>MNHKVHHHHHHMELGTLEGSENLYFQGAMARGVNKVILIGNLGDKPELRYTGSGTAVCNMS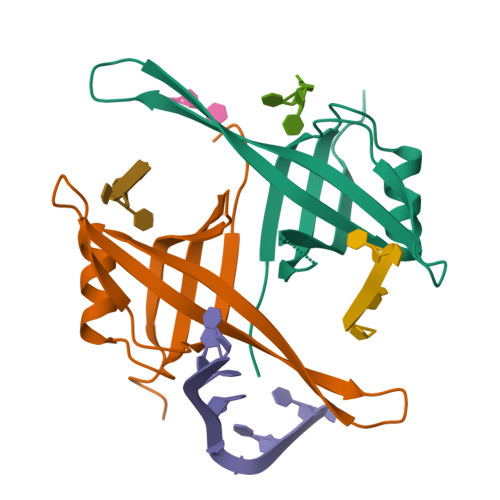LATNETYTDSDGNEVQNTEWHDVVAWGRLGEICNEYLKKGSQVYFEGKLQTRSWEDRDNNTRYSTEVKAQEMMFLDSNRQGGADMDGFDQTRGDESLDQTRQEQPAGSSGPQPGQQASSGGEDEDTFEPDDDLPF[2x]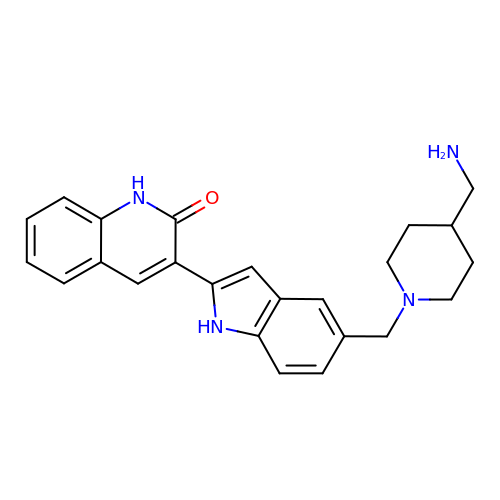3-(5-{[4-(AMINOMETHYL)PIPERIDIN-1-YL]METHYL}-1H-INDOL-2-YL)QUINOLIN-2(1H)-ONE | C24 H26 N4 O | KBIHHEGEALBUMT-UHFFFAOYSA-N>[20x]GHMSDLVTKFESLIISK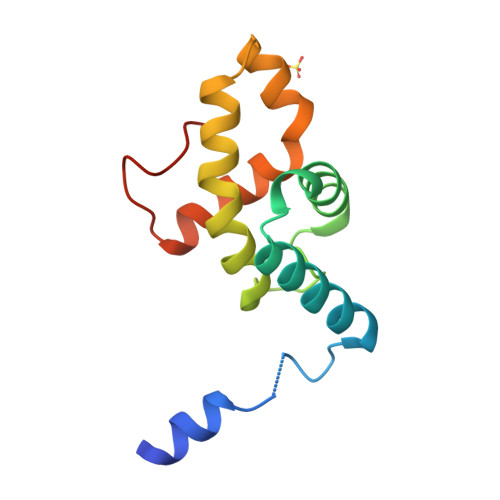YPVSFTKEQSAQAAQWESVLKSGQIQPHLDQLNLVLRDNTFIVSTLYPTSTDVHVFEVALPLIKDLVASSKDVKSTYTTYRHILRWIDYMQNLLEVSSTDKLEINHD> MLRKDIGIDLGTANTLVFLRGKGIVVNEPSVIAIDSTTGEILKVGLEAKNMIGKTPATIKAIRPMRDGVIADYTVALVMLRYFINKAKGGMNLFKPRVVIGVPIGITDVERRAILDAGLEAGASKVFLIEEPMAAAIGSNLNVEEPSGNMVVDIGGGTTEVAVISLGSIVTWESIRIAGDEMDEAIVQYVRETYRVAIGERTAERVKIEIGNVFPSKENDELETTVSGIDLSTGLPRKLT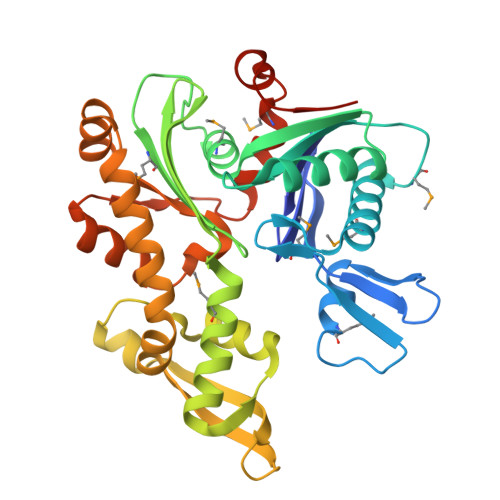LKGGEVREALRSVVVAIVESVRTTLEKTPPELVSDIIERGIFLTGGGSLLRGLDTLLQKETGISVIRSEEPLTAVAKGAGMVLDKVNILKKLQGAGGSHHHHHH> PISPIETVPVKLKPGMDGPKVKQWPLTEEKIKALVEICTEMEKEGKISKIGPENPYNTPVFAIKKKDSTKWRKLVDFRELNKRTQDFWEVQLGIPHPAGLKKKKSVTVLDVGDAYFSVPLDEDFRKYTAFTIPSINNETPGIRYQYNVLPQGWKGSPAIFQSSMTKILEPFAAQNPDIVIYQYMDDLYVGSDLEIGQHRTKIEELRQHLLRWGLTTPDKKHQKEPPFLWMGYELHPDKWTVQPIVLPEKDSWTVNDIQKLVGKLNWASQIYPGIKVRQLSKLLRGTKALTEVIPLTEEAELELAENREILKEPVHGVYYDPSKDLIAEIQKQGQGQWTYQIYQEPFKNLKTGKYARMRGAHTNDVKQLTEAVQKITTESIVIWGKTPKFKLPIQKETWETWWTEYWQATWIPEWEFVNTPPLVKLWYQLEKEPIVGAETFYVDGAANRETKLGKAGYVTNKGRQKVVPLTNTTNQKTELQAIYLALQDSGLEVNIVTDSQYALGIIQAQPDKSESELVNQIIEQLIKKEKVYLAWVPAHKGIGGNEQVD;> PISPIETVPVKLKPGMDGPKVKQWPLTEEKIKALVEICTEMEKEGKISKIGPENPYNTPVFAIKKKDSTKWRKLVDFRELNKRTQDFWEVQLGIPHPAGLKKKKSVTVLDVGDAYFSVPLDEDFRKYTAFTIPSINNETPGIRYQYNVLPQGWKGSPAIFQSSMTKILEPFKKQNPDIVIYQYMDDLYVGSDLEIGQHRTKIEELRQHLLRWGLTTPDKKHQKEPPFLWMGYELHPDKWTVQPIVLPEKDSWTVNDIQKLVGKLNWASQIYPGIKVRQLSKLLRGTKALTEVIPLTE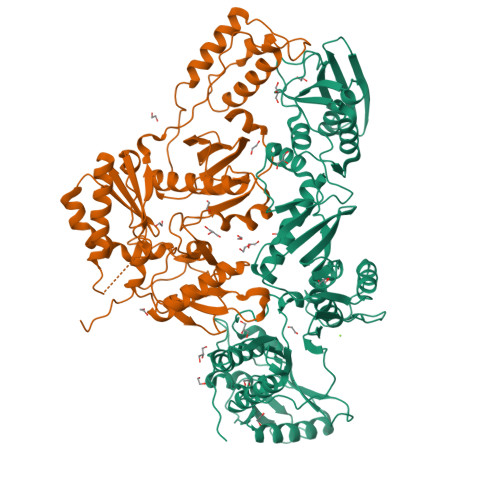EAELELAENREILKEPVHGVYYDPSKDLIAEIQKQGQGQWTYQIYQEPFKNLKTGKYARMRGAHTNDVKQLTEAVQKITTESIVIWGKTPKFKLPIQKETWETWWTEYWQATWIPEWEFVNTPPLVKLWY Signals are initiated by extracellular interactions of the Notch receptor with Delta/Serrate/Lag-2 (DSL) ligands, whose structure is highly conserved throughout evolution. Here, we demonstrate that the N terminus of human Jagged-1 is a C2 phospholipid recognition domain that binds phospholipid bilayers in a calcium-dependent fashion. We expressed and solved the structure of a Notch ligand fragment consisting of the full N-terminal extension, the Notch-binding DSL domain, and the three adjacent EGF domains from human Jagged-1 (J-1N-EGF3). Our structure demonstrates that the N-terminal portion of Jagged-1 folds as a C2-phospholipid-recognition domain with strong structural, but not sequence, homology to the Munc13 C2B domain (root-mean-square deviation [rmsd] 2.7 Å versus Protein Data Bank 3KWT, 10% sequence identity; Figure 1B; Cho and Stahelin, 2006; Shin et al., 2010).

To explore the molecular basis of the effects of this double mutant, we determined the J-1N-EGF3 structure from crystals grown at a physiological pH in the presence of 7.5 mM Ca2+. These crystals contain two independent copies of J-1N-EGF3, and, as observed for other Ca2+-dependent C2 domains, Ca2+ is seen to bind in a cleft between the β1-β2 and β5-β6 loops at the top of the C2 domain, ordering them despite the increased length of these loops in Jagged-1 compared with other C2 domains. The observed bidentate coordination of the bound Ca2+ by Asp140 suggests that it is substitution of this side chain by Ala in the D140A/D144A mutant that explains the loss of Ca2+ binding as shown by increased proteolytic susceptibility, reduced Tm, and significantly reduced phospholipid binding. It is noteworthy that even in the presence of Ca2+ at concentrations that our thermal denaturation assay suggests would be fully saturating, the β5-β6 and β1-β2 loops remain highly mobile, with their conformations varying between the two crystallographically independent copies of the molecule.

>[2x]SGQFELEILSMQNVNGELQNGNCCGGARNPGDRKCTRDECDTYFKVCLKEYQSRVTAGGPCSFGSGSTPVIGGNTFNLKASRGNDRNRIVLPFSFAWPRSYTLLVEAWDSSNDTVQPDSIIEKASHSGMINPSRQWQTLKQNTGVAHFEYQIRVTCDDYYYGFGCNKFCRPRDDFFGHYACDQNGNKTCMEGWMGPECNRAICRQGCSPKHGSCKLPGDCRCQYGWQGLYCDKCIPHPGCVHGICNEPWQCLCETNWGGQLCDKDLNYCGTHQPCLNGGTCSNTGPDKYQCSCPEGYSGPNCEIVDHHHHHH>[4x]MAIDLRPFIPFGRGALSQATDPFRAAVEFTLMPMLITNPHLPDNPIVFANPAFLKLTGYEADEVMGRNCRFLQGHGTDPAHVRAIKSAIAAEKPIDIDIINYKKSGEAFWNRLHISPVHNANGRLQHFVSSQLDVTLELSRLVELEKERKTLSIETARSKDQLDYIVEVANIGFWTREFYSGKMTCSAECRRIYGFTPDEPVHFDTILDLVVLEDRMTVVQKAHQAVTGEPYSIEYRIVTRLGETRWLETRAKALTGENPLVLGIVQDVTERKHHHHHH

LOV-HK is a blue light photoreceptor from Brucella abortus, a pathogenic α-2-proteobacterium that can be transmitted from cattle to humans causing brucellosis. B. abortus LOV-HK comprises an N-terminal blue light-sensing LOV domain, a central PAS (Per-Arnt-Sim) domain of unknown function and a C-terminal HK domain. The LOV and PAS domains are connected through a long linker helix denoted the Jα helix, while the HK domain belongs to the HWE family. Upon blue light illumination, B. abortus LOV-HK photobleaches as a result of the adduct formation between its flavin mononucleotide (FMN) chromophore and an adjacent conserved cysteine residue as in other LOV proteins.

To address whether these differences are indeed light-induced structural changes or whether they are simply due to different constructs crystallized under different conditions, we conducted dynamic crystallographic experiments to examine the light-induced structural changes in the photoactive LOV-PAS crystals. We collected 22 crystallographic data sets by subjecting the LOV-PAS crystals to various dark and light conditions at room temperature before freezing. Although the dark and light crystals belong to the same space group, they show small yet consistent differences in their cell parameters. In the light LOV-PAS structure, all four subunits exhibit the tilting of FMN toward the Eα helix forming stronger H-bonds with Gln132. It is highly possible that the FMN tilting results from the widely reported light-induced adduct formation between the FMN-C4a and Cys69-Sγ atoms, which is not fully resolved in our electron density maps. In addition to the FMN tilting, the LOV domain moves concertedly as a rigid body in response to light. Specifically, the LOV domains undergo partial separation across the dimer interface in both the AB and CD dimers, which is also evidenced by the increased intersubunit distances in the light-minus-dark difference distance matrices. Partial separation between the LOV domains results in a destabilized or altered dimer interface between the N-terminal parts of the Jα helices. Instead of moving with their respective LOV domains, the tethered Jα helices in both the AB and CD dimers move together sideways perpendicular to the helical spine, resulting in asymmetric responses between the partner subunits. Although these motions observed in the LOV-PAS crystals are small in amplitude due to lattice restraints, they are compatible with the Jα tilting captured by the light LOV-PAS-HK structure, where the helical tilting is coupled to unwinding of the helical spine, eventually leading to a large rotation of the PAS dimer relative to the LOV dimer.> MVPISPIETVPVKLKPGMDGPKVKQWPLTEEKIKALVEICTEMEKEGKISKIGPENPYNTPVFAIKKKDSTKWRKLVDFRELNKRTQDFWEVQLGIPHPAGLKQKKSVTVLDVGDAYFSVPLDKDFRKYTAFTIPSINNETPGIRYQYNVLPMGWKGSPAIFQCSMTKILEPFRKQNPDIVIYQYMDDLYVGSDLEIGQHRTKIEELRQHLLRWGFTTPDKKHQKEPPFLWMGYELHPDKWTVQPIVLPEKDSWTVNDIQKLVGKLNWASQIYAGIKVRQLCKLLRGTKALTEVVPLTEEAELELAENREILKEPVHGVYYDPSKDLIAEIQKQGQGQWTYQIYQEPFKNLKTGKYARMKGAHTNDVKQLTEAVQKIATESIVIWGKTPKFKLPIQKETWEAWWTEYWQATWIPEWEFVNTPPLVKLWYQLEKEPIIGAETFYVDGAANRETKLGKAGYVTDRGRQKVVPLTDTTNQKTELQAIHLALQDSGLEVNIVTDSQYALGIIQAQPDKSESELVSQIIEQLIKK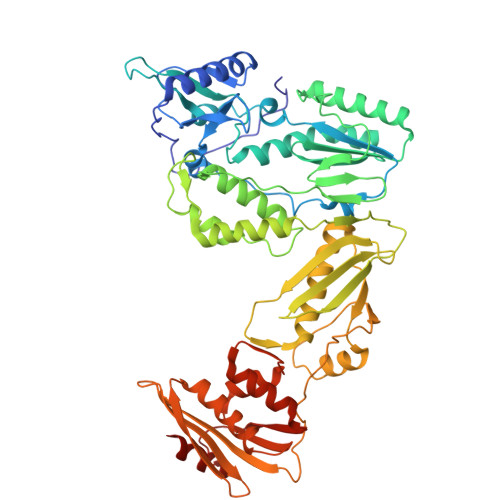EKVYLAWVPAHKGIGGNEQVDKLVSAGIRKVL> RGSATDTAATTGTASPDEPLYVQGQTELDDVTSDNDVVLADFYADWCG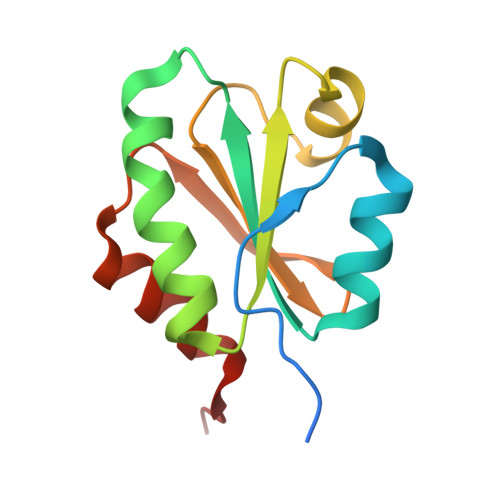PCQMLEPVVETLAEQTDAAVAKIDVDENQALASAYGVRGVPTLVLFADGEQVEEVVGLQDEDALKDLIESYTELVP>[2x]EVSQDLFNQFNLFAQYSAAAYCGKNNDAPAGTNITCTGNACPEVEKADATFLYSFEDSGVGDVTGFLALDNTNKLIVLSFRGSRSIENWIGNLNFDLKEINDICSGCRGHDGFTSSWRSVADTLRQKVEDAVREHPDYRVVFTGHSLGGALATVAGADLRGNGYDIDVFSYGAPRVGNRAFAEFLTVQTGGTLYRITHT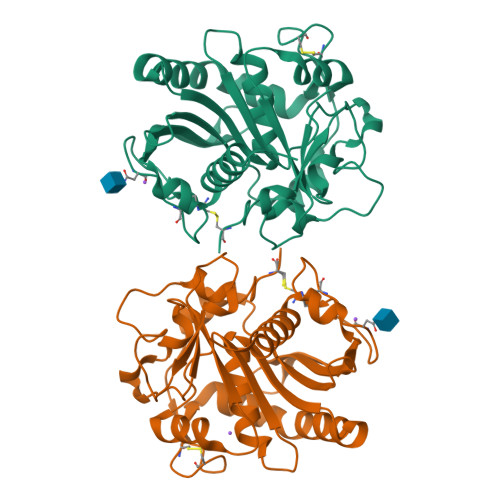NDIVPRLPPREFGYSHSSPEYWIKSGTLVPVTRNDIVKIEGIDATGGNNQPNIPDIPAHLWYFGLIGTCL> KDTIALVVSTLNNPFFVSLKDGAQKEADKLGYNLVVLDSQNNPAKELANVQDLTVRGTKILLINPTDSDAVDNAVKMANQANIPVITLDRQATKGEVVSHIASDNVLGGKIAGDYIAKKAGEGAKVIELQGIAGTSAARERGEGFQ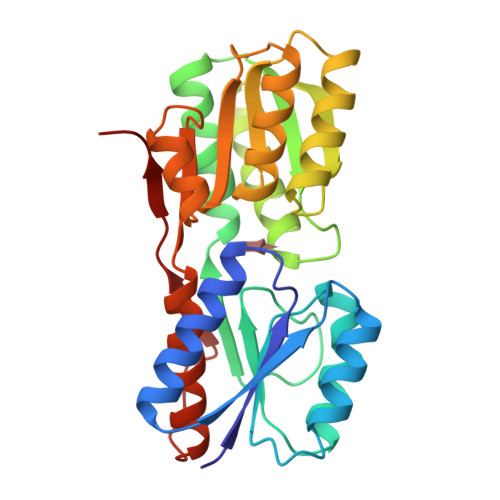QAVAAHKFNVLASQPADFDRIKGLNVMQNLLTAHPDVQAVFAQNDEMALGALRALQTAGKSDVMVVGFDGTPDGEKAVNDGKLAATIAQLPDQIGAKGVETADKVLKGEKVQAKYPVDLKLVVKQ3-chloro-5-{4-chloro-2-[2-(5-chloro-2,4-dioxo-3,4-dihydropyrimidin-1(2H)-yl)ethoxy]phenoxy}benzonitrile | C19 H12 Cl3 N3 O4 | 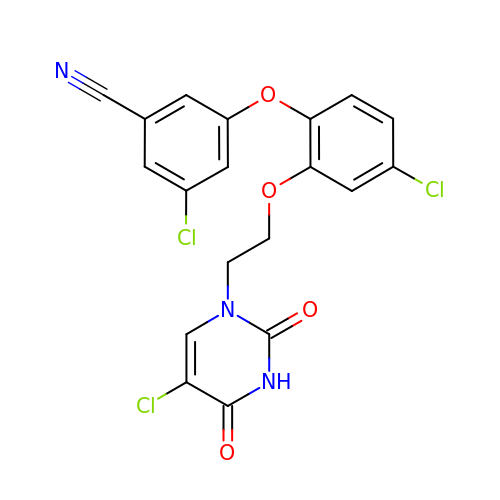MPBULEIWOAXAKX-UHFFFAOYSA-N> SKKQDENIVVNKFKPKEPYVGRCLLNTKITGDDAPGETWHMVFSTEGEVPYREGQSIGIVPDGIDKNGKPHKLRLYSIASSAIGDFGDSKTVSLCVKRLVYTNDAGEVVKGVCSNFLCDLKPGSEVKITGPVGKEMLMPKDPNATVIMLGTGTGIAPFRSFLWKMFFEKHEDYQFNGLAWLFLGVPTSSSLLYKEEFEKMKEKAPENFRLDFAVSREQVNDKGEKMYIQTRMAQYAEELWELLKKDNTFVYMCGLKGMEKGIDDI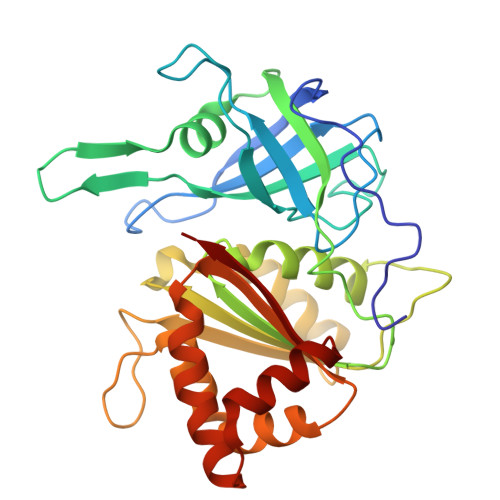MVSLAAKDGIDWIEYKRTLKKAEQWNVEVYL> MKTVLIGVGQAGGKLASALQSFDRQTGFGAVLDAVAVNTAKADLQSLPVETVLIGQDRVNGHGVGGDNELGAAVMESDQTEVMSALDGRVTAEAESIFVVAGLGGGSGSGGAPVLAKALAGVYDVPVYVLGILPGADEGALYQVNAGRSLKTVAREADAVLLVDNDAFRSAGESMSEGYDAINEAIARRVGLLLAAGEATEGVGESVVDTSEVINTLRSGGIAALGYASAEASPNAEDNINAVMSTTRRAVLTGTSLPDASDADAALVVIAGEPDTIPRKGVERARRWVEDETGSMQVRGGDFPLESGRLASLVLLGGVERSERVE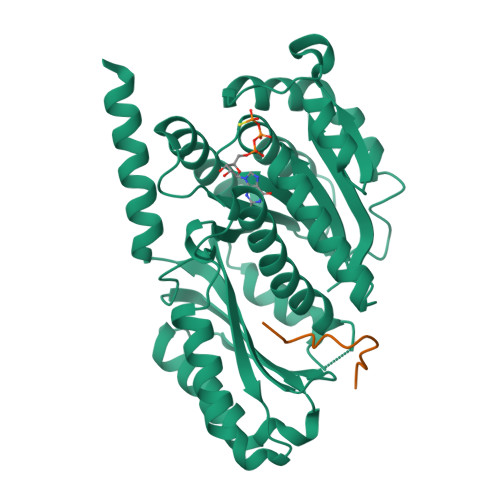SFMERAREAIDKAETEPREDPKG;> MWHSDDLDDLLGSHHHHHH>[2x]GELVRTDSPNFLCSVLPTHWRCNKTLPIAFKVVAKGDVPDGTLVTVMAGNDENYSAELRNATAAMKNQVARFNDLRFVGRSGRGKSFTLTITVFTNPPQVATYHRAIAITVDGPREPRRHRQKLDDQTKPGSLSFSERLSELEQLRRTAMRVSPHHPAPTPNPRASLNHSTAFNPQPQSQMQDARQIQPSPPWSYDQSYQYLGS;>MPRVVPDQRSKFENEEFFRKLSRECEIKYTGFRDRPHEERQTRFQNACRDGRSEIAFVATGTNLSLQFFPASWQGEQRQTPSREYVDLEREAGKVYLKAPMILNGVCVIWKGWIDLHRLDGMGCLEFDEERAQQEDALAQQA[2x];>SLQRVPSYDSFDSEDYPAALPNHKPKGTFKDYVRDRADLNKDKPVIPAAALAGYTGSGPIQLWQFLLELLTDKSC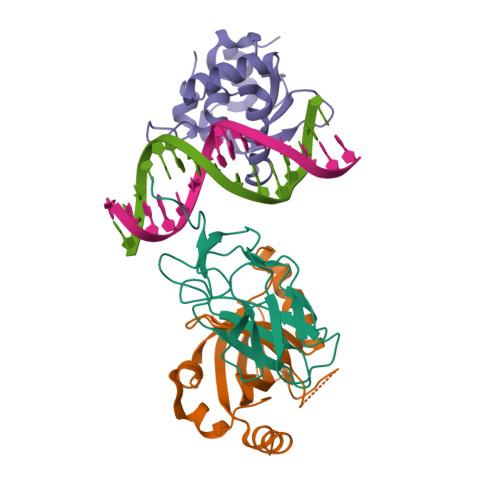QSFISWTGDGWEFKLSDPDEVARRWGKRKNKPKMNYEKLSRGLRYYYDKNIIHKTAGKRYVYRFVCDLQSLLGYTPEELHAMLDVKPDADE[2x]> NDPIANAVESAVSALADTTISRVTAANTTASTHSLGTGRVPALQAAETGASSNASDENLVETRCVMNRNGVNEASVEHFYSRAGLVGVVEVKDSGTSLDGYTVWPIDVMGFVQQRRKLELSTYMRFDAEFTFVSNLSNSTTPGMLLQYMYVPPGAPKPDGRKSYQWQTATNPSVFAKLSDPPPQVSVPFMSPATAYQWFYDGYPTFGEHKQATNLQYGQCPNNMMGHF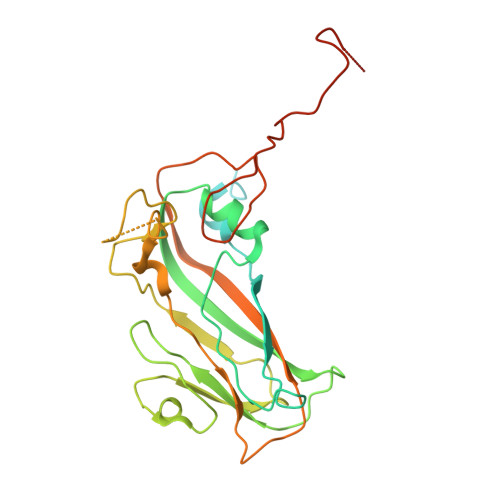AIRTVSESTTGKNVHVRVYMRIKHVRAWVPRPLRSQAYMVKNYPTYSQTITNTATDRASITTTDYEGGVPASPQRTS> MAGRQSHKKIDVRNDTSTRYKGKLYGIFVNYMGE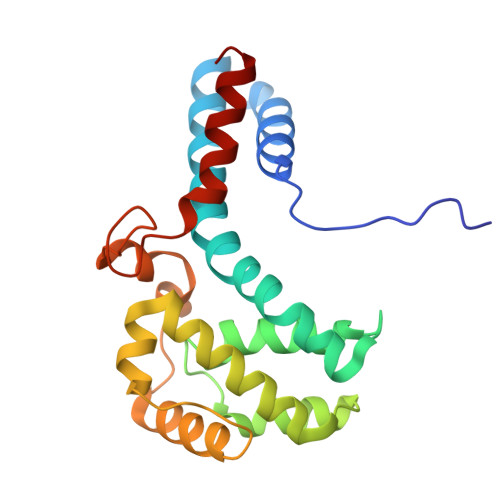KYAQQLVENMYSNYNDVFVEIYNKMHNALRPTLVKLAGAGATFPLWQLVNEAIYAVYLTHKETASFLVTKYVARGVPAMTVKTLLAEVGNQLKELVPAVAEQIGSVTLDHTNVVSTVDNIVTSMPALPNSYAGVLMKTKVPTVTPHYAGTGTFSSMESAYKALEDIERGL TRIBROMOMETHANE 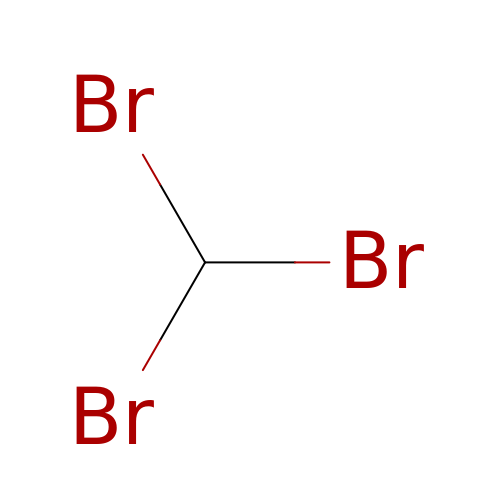| C H Br3 | DIKBFYAXUHHXCS-UHFFFAOYSA-N>[11x]MSGRWSHPQFEKVNDPPVPALLWAQEVGQVLAGRARRLLLQFGVLFCTILLLLWV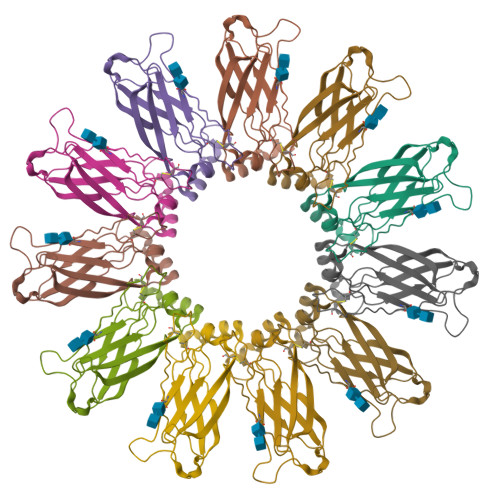SVFLYGSFYYSYMPTVSHLSPVHFYYRTDCDSSTTSLCSFPVANVSLTKGGRDRVLMYGQPYRVTLELELPESPVNQDLGMFLVTISCYTRGGRIISTSSRSVMLHYRSDLLQMLDTLVFSSLLLFGFAEQKQLLEVELYADYRENSYVPTTGAIIEIHSKRIQLYGAYLRIHAHFTGLRYLLYNFPMTCAFIGVASNFTFLSVIVLFSYMQWVWGGIWPRHRFSLQVNIRKRDNSRKEVQRRISAHQPGPEGQEESTPQSDVTEDGESPEDPSGTEGQLSEEEKPDQQPLSGEEELEPEASDGSGSWEDAALLTEANLPAPAPASASAPVLETLGSSEPAGGALRQRPTCSSS>[4x]SNAMSMAYEEYMRQLVVPMRRELTGAGFEELTTAEEVENFMEKAEGTTLVVVNSVCGCAAGLARPAAT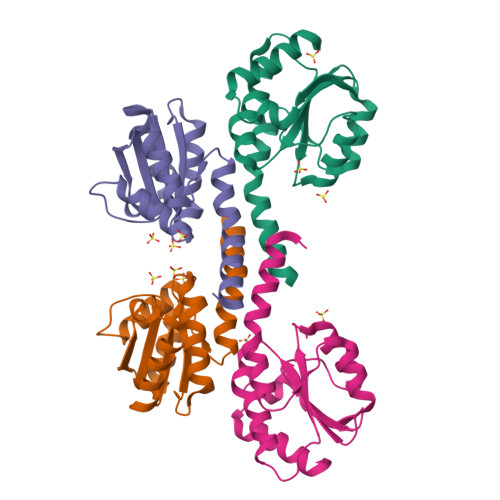QAVLQNDKTPDNTVTVFAGQDKEATAKMREYFTGAAPSSPSMALLKGKEVVHFIPRHEIEGHDMEEIMKNLTAAFDAHC>GPLGSMQNSHMEE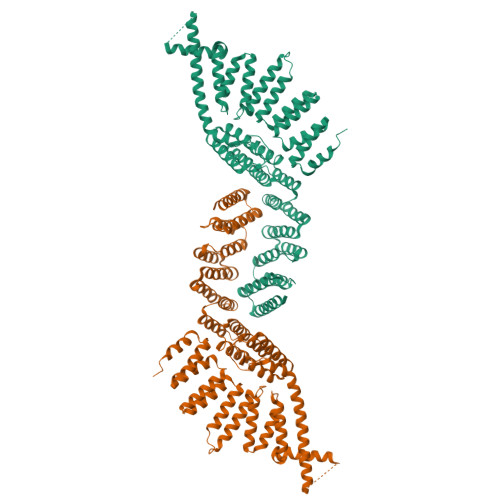YRNSDNGSTGNSSEVAVVEHPDFSTEIMNVTEMEQSPDASPSAHASTEENEMANAVNLPVTEAEGDFPPEFEKFWKTVEMNPQDFTGWVYLLQYVEQENHLMAARKAFDKFFVHYPYCYGYWKKYADLEKRHDNIKQSDEVYRRGLQAIPLSVDLWIHYINFLKETLDPGDQETNTTIRGTFEHAVLAAGTDFRSDKLWEMYINWENEQGNLREVTAVYDRILGIPTQLYSHHFQRFKEHVQNNLPRDLLTGEQFIQLRRELASVNGHSGDDGPPGDDLPSGIEDITDPAKLITEIENMRHRIIEIHQEMFNYNEHEVSKRWTFEEGIKRPYFHVKPLEKAQLKNWKEYLEFEIENGTHERVVVLFERCVISCALYEEFWIKYAKYMENHSIEGVRHVFSRACTVHLPKKPMAHMLWAAFEEQQGNINEARIILRTFEECVLGLAMVRLRRVSLERRHGNMEEAEHLLQDAIKNAKSNNESSFYAIKLARHLFKIQKNLPKSRKVLLEAIEKDKENTKLYLNLLEMEYSCDLKQNEENILNCFDKAIHGSLPIKMRITFSQRKVEFLEDFGSDVNKLLNAYDEHQTLLKEQDTLKRKAENGSEEPEEKKAHTEDLSSAQIIDGDLQANQAAYNYSAWYQYNYQNPWNYGQYYPPPPT[2x]> GAMGSDEEQSPDWDSHGLPANIVVQLNKLSGFKKYKVSDIMFFDRRRQTTIGTEDSFFEMVSIRPGGVYTKAQLQKELETLATCGMFEKVDLEGKTKPDGTLGVTISFAESTWQSADRF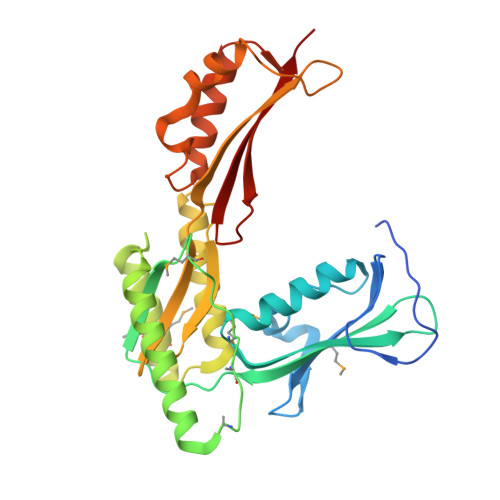RCINVGLMVQSKPIEMDSDMTDKEKLEYYRSLEKDYKRRIDRARPCLLPAPVYGEVMQMLRDQGKVSARLLQRIRDRVQKWYHDEGYACAQVVNFGNLNTKEVVCEVVEGDITQLVIQFQDKLGNVVEGNTQVPVVRRELPKQLRQGYVFNIEAGKKALSNINSLGLFSNIEVNPRPDEKNEGGIIVEIKLKELE>GMETVQLRNPPRRQLKKLDEDSLTKQPEEVFDVLEKLGEGSYGSVYKAIHKETGQIVAIKQVPVESDLQE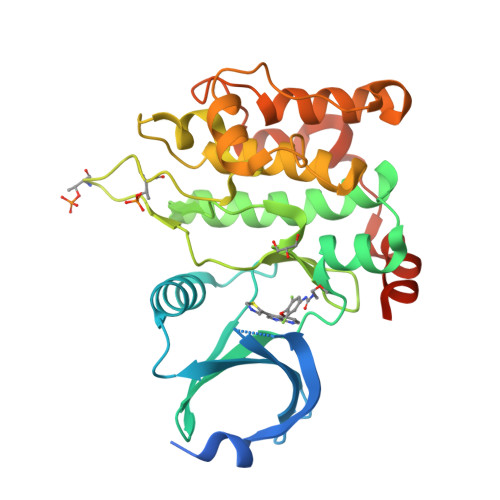IIKEISIMQQCDSPHVVKYYGSYFKNTDLWIVMEYCGAGSVSDIIRLRNKTLTEDEIATILQSTLKGLEYLHFMRKIHRDIKAGNILLNTEGHAKLADFGVAGQLTDTMAKRNTVIGTPFWMAPEVIQEIGYNCVADIWSLGITAIEMAEGKPPYADIHPMRAIFMIPTNPPPTFRKPELWSDNFTDFVKQCLVKSPEQRATATQLLQHPFVRSAKGVSILRDLINEAMDVKLKRQESQQRE[2x]> MGLEKTVKEKLSFEGVGIHTGEYSKLIIHPEKEGTGIRFFKN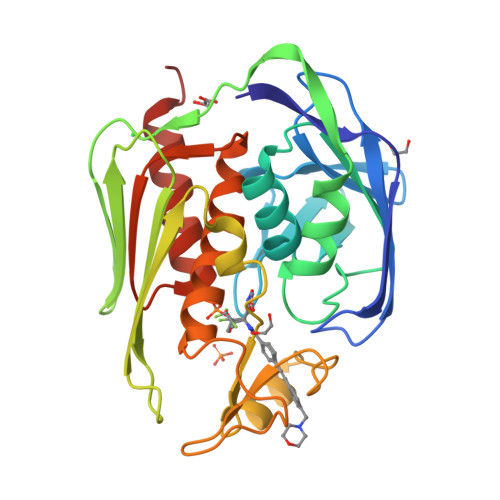GVYIPARHEFVVHTNHSTDLGFKGQRIKTVEHILSVLHLLEITNVTIEVIGNEIPILDGSGWEFYEAIRKNILNQNREIDYFVVEEPIIVEDEGRLIKAEPSDTLEVTYEGEFKNFLGRQKFTFVEGNEEEIVLARTFAFDWEIEHIKKVGLGKGGSLKNTLVLGKDKVYNPEGLRYENEPVRHKVFDLIGDLYLLGSPVKGKFYSFRGGHSLNVKLVKELAKKQKLTRDLPH N-{[2-(naphthalen-2-yl)-1,3-thiazol-4-yl]acetyl}glycine | C17 H14 N2 O3 S | 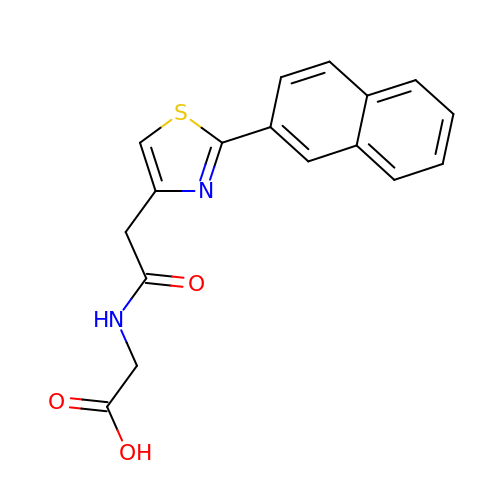VQPWBMLXWGTCAU-UHFFFAOYSA-N> QSSVTLFGIVDTNVAYVNKDAAGDSRYGLGTSGASTSRLGLRGTEDLGGGLKAGFWLEGEIFGDDGNASGFNFKRRSTVSLSGNFGEVRLGRDLVPTSQKLTSYDLFSATGIGPFMGFRNWAAGQGADDNGIRANNLISYYTPNFGGFNAGFGYAFDEKQTIGTADSVGRYIGGYVAYDNGPLSASLGLAQQKTAVGGLATDRDEITLGASYNFGVAKLSGLLQQTKFKRDIGGDIKTNSYMLGASAPVGGVGEVKLQYALYDQKAIDSKAHQITLGYVHNLSK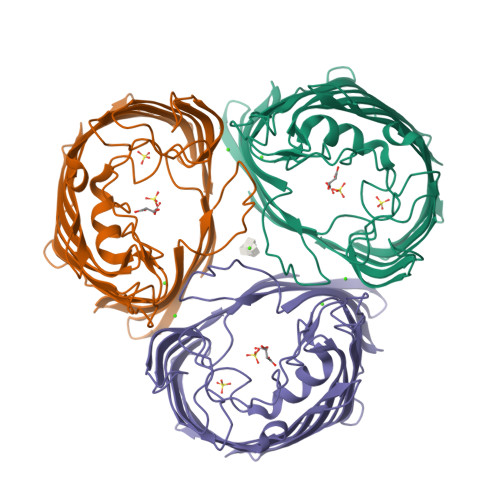RTALYGNLAFLKNKDASTLGLQAKGVYAGGVQAGESQTGVQVGIRHAF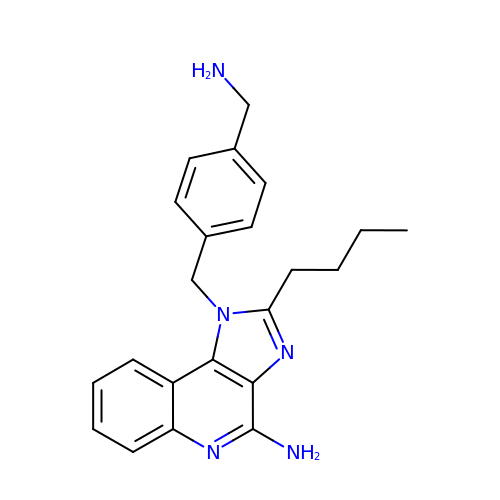1-[[4-(aminomethyl)phenyl]methyl]-2-butyl-imidazo[4,5-c]quinolin-4-amine | C22 H25 N5 | SDSKFWHQCNBICO-UHFFFAOYSA-N> GPGPEIVDTCSLASPASVCRTKHLHLRCSVDFTRRTLTGTAALTVQSQEDNLRSLVLDTKDLTIEKVVINGQEVKYALGERQSYKGSPMEISLPIALSKNQEIVIEISFETSPKSSALQWLTPEQTSGKEHPYLFSQCQAIHCRAILPCQDTPSVKLTYTAEVSVPKELVALMSAIRDGETPDPEDPSRKIYKFIQKVPIPCYLIALVVGALESRQIGPRTLVWSEKEQVEKSAYEFSETESMLKIAED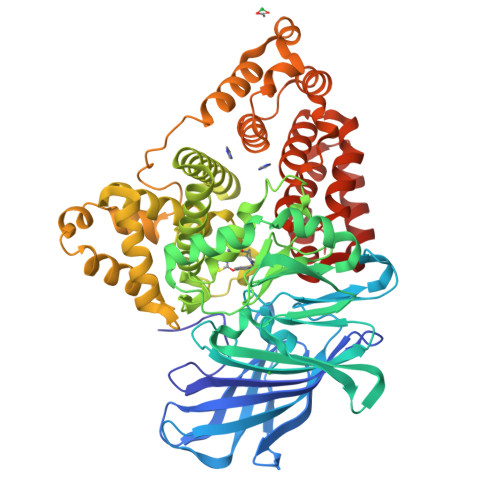LGGPYVWGQYDLLVLPPSFPYGGMENPCLTFVTPTLLAGDKSLSNVIAHEISHSWTGNLVTNKTWDHFWLNEGHTVYLERHICGRLFGEKFRHFNALGGWGELQNSVKTFGETHPFTKLVVDLTDIDPDVAYSSVPYEKGFALLFYLEQLLGGPEIFLGFLKAYVEKFSYKSITTDDWKDFLYSYFKDKVDVLNQVDWNAWLYSPGLPPIKPNYDMTLTNACIALSQRWITAKEDDLNSFNATDLKDLSSHQLNEFLAQTLQRAPLPLGHIKRMQEVYNFNAINNSEIRFRWLRLCIQSKWEDAIPLALKMATEQGRMKFTRPLFKDLAAFDKSHDQAVRTYQEHKASMHPVTAMLVGKDLKVD> GSHMDFVAFMNKINSINANLSRYENIINQIDAQHKDLLTQVSEEQEMELRRSLDDYISQATDLQYQLKADIKDAQRDGLHDSNKQAQAENCRQKFLKLIQDYRIIDSNYKEESKEQAKRQYTIIQPEATDEEVEAAI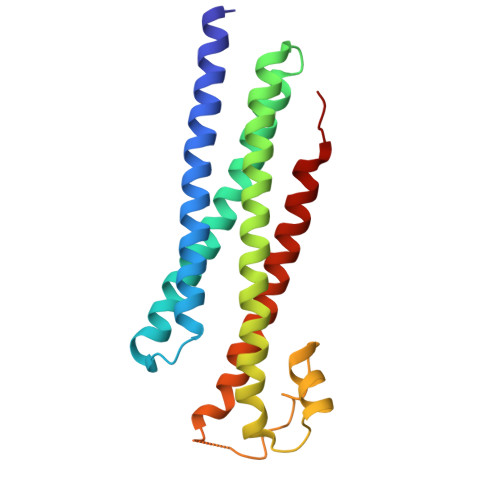NDVNGQQIFSQALLNANRRGEAKTALAEVQARHQELLKLEKTMAELTQLFNDMEELVIE>DKNIIIGAMTALITPFKNGKVDEQSYARLIKRQIENGIDAVVPVGTTGESATLTHEEHRTCIEIAVETCKGTKVKVLAGAGSNATHEAVGLAKFAKEHGADGILSVAPYYNKPTQQGLYEHYKAIAQSVDIPVLLYNVPGRTGCEISTDTIIKLFRDCEN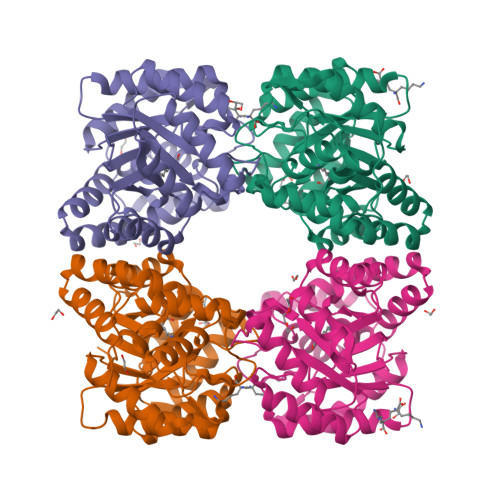IYGVKEASGNIDKCVDLLAHEPRMMLISGEDAINYPILSNGGKGVISVTSNLLPDMISALTHFALDENYKEAKKINDELYNINKILFCESNPIPIKTAMYLAGLIESLEFRLPLCSPSKENFAKIEEVMKKYKIKGF[4x]> SFGDGF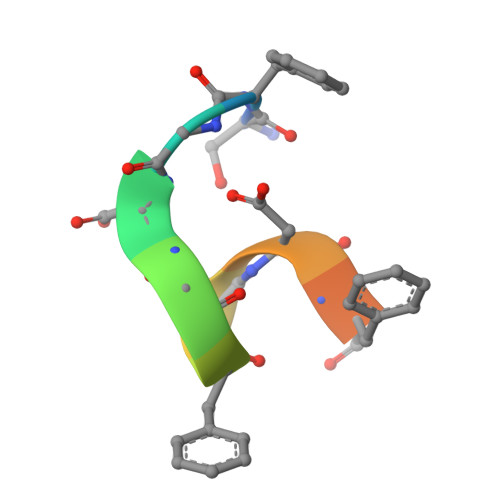ADFSTL>LTPKETCDLCQIALRTVFGHFGGNIPSRRKLVHQLKHECKRHFNYRRRCLLLMKVNSDLIFREMTDGSFKPMEVCLIMRECNPHDSPLEPEMIDKSGQPEAFALVSSSDDNYDTSEE[2x]

In this study, we investigate the structure and biochemical functions of two SAPLIPs from human (Necator americanus) and dog hookworm (Ancylostoma caninum), Na-SLP-1 and Ac-SLP-1. The structure of both hookworm SAPLIPs were determined in hexagonal space groups, and closely resemble the fold of the Sap domain, as known from saposins and other SAPLIPs. The fold is comprised of a four- or five-helix bundle, where a kink in the third helix can lead to occurrence of two helices, α3 and α4. Three conserved dithioether bonds link helix α1 with the C-terminal end, helices α1 and α5, and helices α2 and α3.

Na-SLP-1, in contrast, is exclusively monomeric (MALS 12970 g/mol; theoretical M = 13530 g/mol). In the crystal structure of Na-SLP-1, the C-terminal extension of about 30 amino acids, which is attached to the N-terminal Sap domain could not be resolved, which agrees with the results from mass spectrometry. The crystal structure contained two molecules in the asymmetric unit, giving rise to a complex network of molecules in the crystal packing with a variety of different protein-protein contacts. The two monomers in the asymmetric unit agree very well in their overall fold as is reflected by the Cα rms deviation of 0.55 Å. The crystal structure of Na-SLP-1 reveals the presence of seven exposed basic residues on helices α2 and α3, giving rise to an extensive basic patch even on one monomer which is likely to initiate contact with the membrane surface, driven by electrostatic interactions. Crystal packing analysis of Na-SLP-1 reveals a P2-symmetric dimer, albeit with a moderate interface area (571 Å2). Despite being a monomeric protein in solution, this dimer may possess a functional importance in the membrane-bound state, since it combines the basic surface clusters of the two monomers into one large patch. For Na-SLP-1, we found 14 void volumes with values larger than 5 Å3, the largest ones being 29 Å3, 30 Å3 and 43 Å3, using the same probe radius as in the granulysin study. Intriguingly, Na-SLP-1 and granulysin share the feature of a loosely packed protein core, as evident from void volumes in the interior of both proteins. The function of Na-SLP-1, in contrast, may be similar to granulysin since both seem to share a scissor-like motion of the two “jaws”.4-[3-[3-[2,4-bis(azanyl)-6-ethyl-pyrimidin-5-yl]prop-2-ynyl]-4-methoxy-phenyl]benzoic acid | C23 H22 N4 O3 | 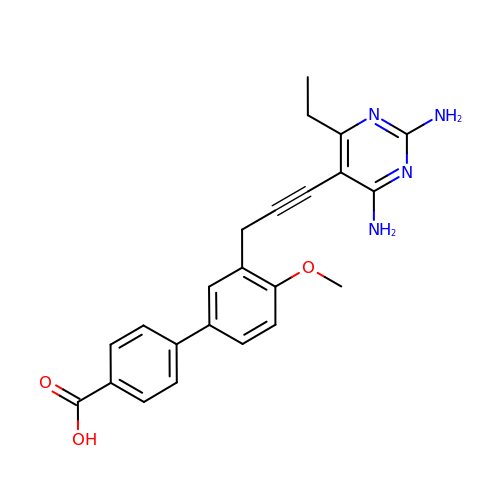KQGRJTMRAQWNLV-UHFFFAOYSA-N>[4x]SNAQETAPFTPDQEKQIENLIHAALFNDPASPRIGAKHPKLTLVNFTDYNCPYCKQLDPMLEKIVQKYPDVAVIIKPLPFKGESSVLAARIALTT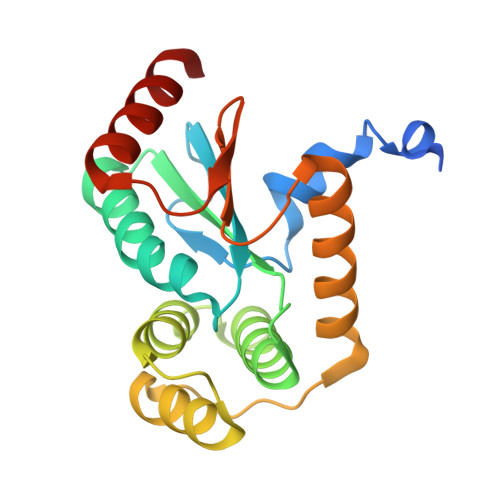WREHPQQFLALHEKLMQKRVYHTDDSIKQAQQKAGATPVTLDEKSMETIRTNLQLARLVGVQGTPATIIGDELIPGAVPWDTLEAVVKEKLASANGG> MDFSRNLYDIGEQLDSEDLASLKFLSLDYIPQRKQEPIKDALMLFQRLQEKRMLEESNLSFLKELLFRINRLDLLITYLNTRKEEMERELQTPGRAQISAYRVMLYQISEEVSRSELRSFKGGLQEEI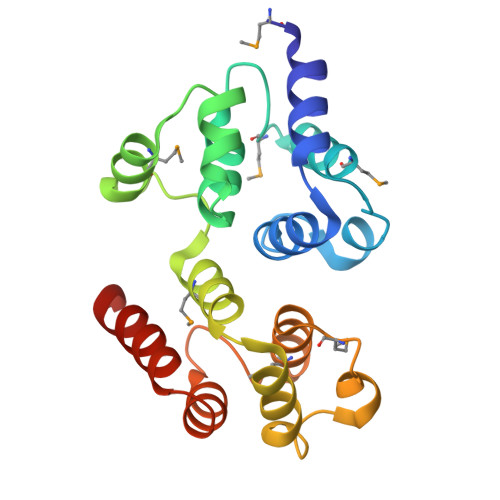SKCKLDDDMNLLDIFIEMEKRVILGEGKLDILKRVCAQINKSLLKIINDYEEFSKER> EELRRRIEELE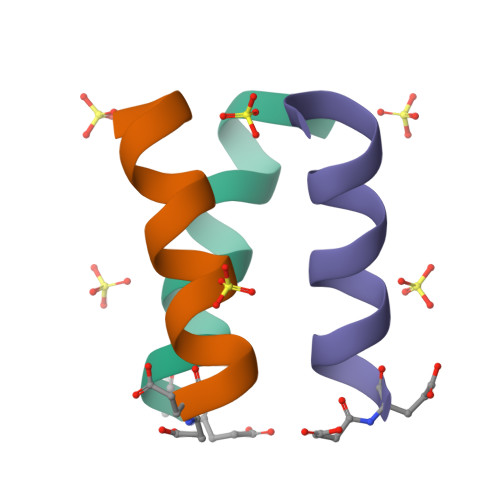RRIRX Galectin (Gal) is a lectin that binds to β-galactosides. Because the primary and tertiary structures of Gal-13 are highly conserved among all galectins, it had been named galectin-13. However, our crystallographic and biochemical experiments (solid phase experiment, hemagglutination assay, and biolayer interferometry) proved that wild-type Gal-13 could not bind lactose or a rhamnogalacturonan Ι domain (RG-I-4) from Ginseng Pectin. Primary structure alignment showed that a highly conserved histidine residue was modified to arginine (Arg53) in the ligand binding site of wild-type Gal-13, which may be why Gal-13 could not bind lactose.

Moreover, in the crystal, Asp33 from one monomer occupies part of the ligand binding site of another Gal-13 monomer. In order to eliminate steric hindrance, this aspartate was mutated to glycine in several variants. All three other variants (R53HH57R, R53HR55NH57R, and R53HR55NR57RD33G) co-crystallized with lactose, but not Tris, even when the crystallization conditions contained 100 mM Tris. This indicates that these three variants prefer to binding lactose. The present results showed that double mutation of R53 to H and H57 to R was sufficient to recover the ability of Gal-13 to bind lactose. However, the pyran surface of the galactose residue in different structures could not be totally merged with each other, and glucose residues showed variable conformations. The conserved tryptophan and histidine residues in the three variants showed the same conformation and position as in Gal-3 and Gal-8N. Arg57 in R53HH57R and R53HH57RD33G showed two different conformations. Arg57 in one conformation could indirectly stabilize the pyran ring of galactose through a water molecule (W).

> SSLPVPYKLPVSLSVGSCVIIKGTPIHSFINGPQLQVDFYTDMDEDSDIAFHFRVRFGNHVVMNRREFGIWMLEETTDYVPFEDGKQFELCIYVHYNEYEIKVNGIRIYGFVHRIPPSFVKMVQVSRDISLTSVCVCN(4S,5R)-4,5-dihydroxy-3-oxocyclohex-1-ene-1-carboxylic 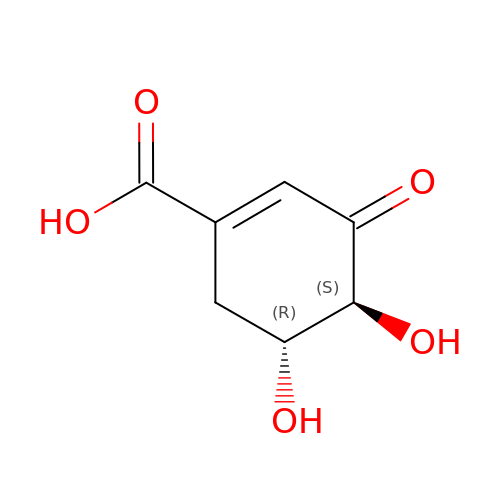acid | C7 H8 O5 | SLWWJZMPHJJOPH-PHDIDXHHSA-N>[4x]GSHMERYDIAIIGSGPAGLASAINAKTRNKSVIVFGSSDLSKKLTLAPVINNYLGFYGIRGAELQEKFKEHIDNMGIQIENVKVNNIYAMGEYFSIMTSKDTYEASKVILAMGMEHTKPLKGEDKFLGRGVGYSATCDAPLYKGKIVTIVGYNKEAESEANYLAELA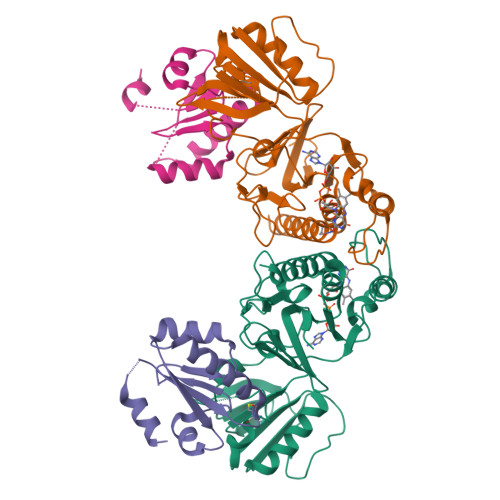SKVYYVPRYKDEYQLVSAVEIVKDVPVEIVGDKKVEKLKLKSRELETDGVFVLKDSAPPEQLVPGLYVEDGHIKVNRKMETNIDGCYAAGDCTGKPYQYMKAVGEGQVAALNAVEKLYTKA;>[4x]GSHMVKEINESIFDEEIKTSGEPVIVDFWAPWCGPSKMLGPIIDELSEDLDGKAKFTKVNVDENPGIASKFGIASIPTVMIFKDGNPVETLVGFRPKQSITASIEKHM> MFENITAAPADPILGLADLFRADERPGKINLGIGVYKDETGKTPVLTSVKKAEQYLLENETTKNYLGIDGIPEFGRCTQELLFGKGSALINDKRARTAQTPGGTGALRVAADFLAKNTSVKRVWVSNPSWPNHKSVFNSAGLEVREYAYYDAENHTLDFDALINSLNEAQAGDVVLFHGCCHAPTGIDPTLEQWQTLAQLSVEKGWLPLFDFAFQGFARGLEEDAEGLRAFAAMHKELIVASSYSKNFGLYNERVGACTLVAA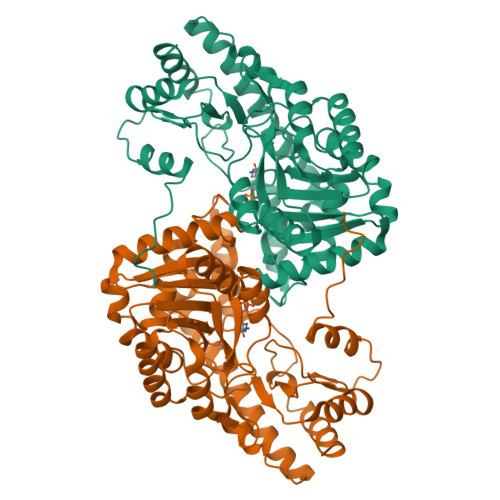DSETVDRAFSQMKAAIRANYSNPPAHGASVVATILSNDALRAIWEQELTDMRQRIQRMRQLFVNTLQEKGANRDFSFIIKQNGMFSFSGLTKEQVLRLREEFGVYAVASGRVNVAGMTPDNMAPLCEAIVAVL>PLGSMENKIVASTKEEFNTWYKQFAEKHKLNNKYTESASFCAEIPQLDTYKYKMELASTDNERDAIYSSALIEATRFCAPIMECAWASCTGTVKRGLEWFDKNKDSDTVKVWDANYQKLRTETPPAEALLAYQKAALNWRKDVGFSIGEYTSILKKAVAAEYKVPGTVINNIKEMLSDMIRRRNRIINGGSDDAPKRGPVGREHLDWCREFASGKFLNAFNPPWGEINKAGKSGYPLLATGLAKLVELEGKDVMDKAKASIAQLEGWVKENKDQVDQDKAEDLLKGVRESYKTALALAKQSNAFRAQGAQIDTVFSSYYWLWKAGVTPVTFPSVSQFLFELGKNPKGQKKMQKALINTPLKWGKRLIELFADNDFTENRIYMHPCVLTSGRMSELGISFGAVPVTSPDDAAQGSGHTKAVLNYKTKTEVGNPCACIISSLFEIQKAGYDIESMDIVASEHLLHQSLVGKRSP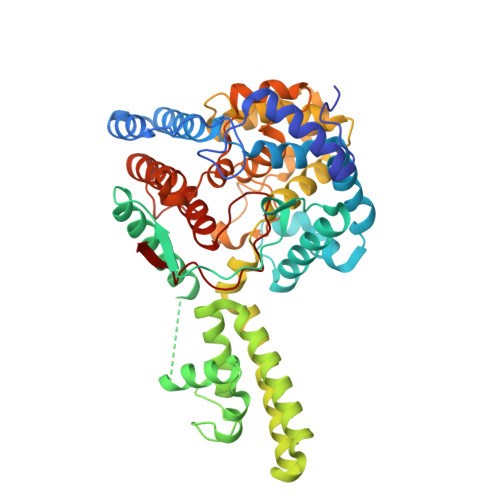FQNAYLIKGNATNINII[4x]4-AMINO-1-BETA-D-RIBOFURANOSYL-2(1H)-PYRIMIDINONE | 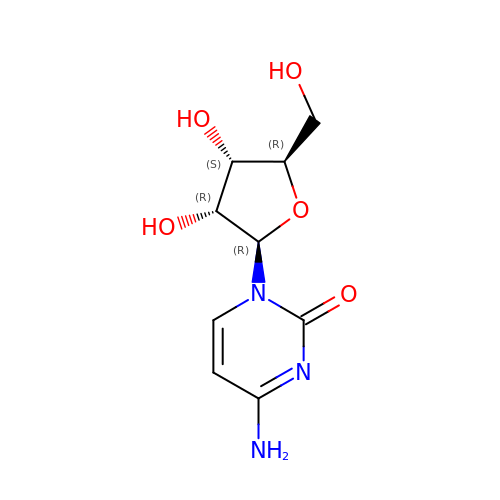C9 H13 N3 O5 | UHDGCWIWMRVCDJ-XVFCMESISA-N2-[2-(2-METHYL-2,3-DIHYDRO-INDOL-1-YL)-2-OXO-ETHYL]-6-MORPHOLIN-4-YL-3H-PYRIMIDIN-4-ONE 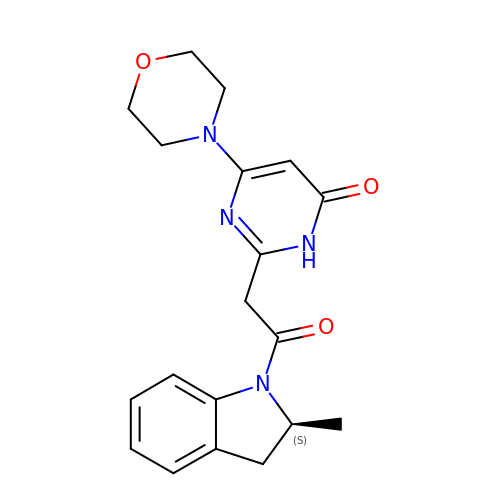| C19 H22 N4 O3 | UAXHPOBBKRWJGA-ZDUSSCGKSA-N>[2x]MIIGYARVSSLDQNLERQLENLKTFGAEKIFTEKQSGKSIENRPILQKALNFVEMGDRFIVESIDRLGRNYNEVIHTVNYLKDKEVQLMITSLPMMNEVTG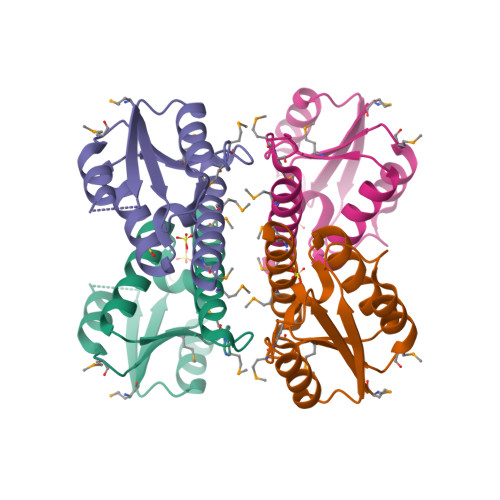NPLLDKFMKDLIIRILAMVSEQERNES Entry of human immunodeficiency virus type 1 (HIV-1) into target cells involves fusion of viral and cellular membranes, a process mediated by the viral surface protein Env (gp160). In the Golgi apparatus, each protomer is cleaved into two subunits that remain noncovalently associated: an N-terminal surface protein (denoted SU or gp120) and a C-terminal transmembrane protein (denoted TM or gp41). Ultimately, the extended state collapses into its most stable form, a trimer-of-hairpins (TOH), in which the C-HR regions pack in an antiparallel manner into hydrophobic grooves on the outside of the N-HR coiled coil. The thermostable core of the gp41 TOH consists of the three-stranded N-HR coiled coil surrounded by three helical C-HR segments.

To determine if asymmetry in TOH structure is a definitive feature of HIV-1 resistance to C37, we also crystallized an N40/C37 construct containing the V549E substitution. Residue 549 (in an e-position of the N-HR hydrophobic heptad repeat) extends directly into the N-HR/C-HR interface where it fills a small hydrophobic pocket bounded by side chains of Asn656, Glu657 and Leu660 and the backbone of the C-HR helix. The six-helix bundle containing the V594E mutation crystallized in a rhombohedral space group (R3) with a defined three-fold crystallographic symmetry down the axis of the N40 coiled coil. The V549E substitution did not disrupt the continuity of the N40 coiled coil nor C37 docking on its surface. Overall, the mutant structure closely resembled the wild type six-helix bundle (RMSD = 0.94 Å). Symmetry dictated that the three C37 peptides bind the V549E-mutant coiled coil with equal affinity, which will be lower than that for the wild type coiled coil due to disrupted hydrophobic packing. Hence, asymmetry is not a general feature of escape from C37-like fusion inhibitors, but rather a special property of the Q552R substitution.

> MQLLSGIEQQQNNLLRAIEAQQHLLQLTVWGIKQLQARILAGGRGGHTTWMEWDREINNYTSLIHSLIEESQNQQEKNEQELLGGHHHHHH>VIKPDPSKYAAEVSTLLTTTWGQQMPYNKLLPKTKKGRLITGCVATATAQVLNYFKYPVRGIGSHTVHYPANDPSGTAISADFGNTTYDWANMKDNYSGNYTEAEANAVATLMLHCGVASEMQYGGPNEGSGAYMTDCAAGLRTYFGFTDAEYITRANYTDEQWMDIVFSELTKGHPLIYGGVSPGSMGQDAGHA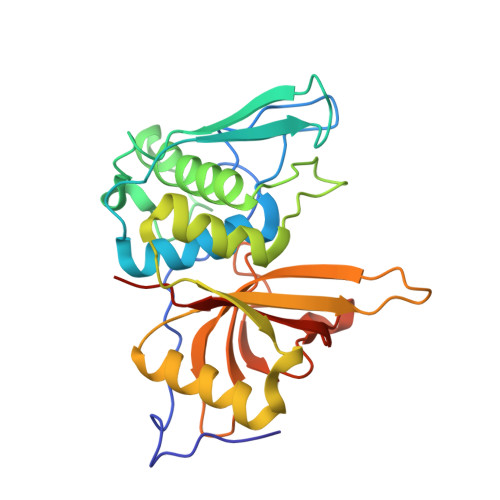FVIDGYNKAGLVSVNWGWNGDVDGYYKIDLLNPGNMYSFTAEQDMVRGVYGKPLED[2x]RIMANTADINE | C12 H21 N | 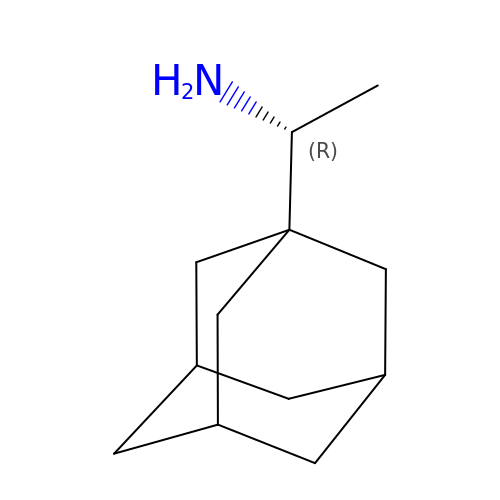UBCHPRBFMUDMNC-RMPHRYRLSA-N N-({(1S)-5-[4-(13-{[2,4-BIS(DIHYDROXYAMINO)PHENYL]AMINO}-2,5,8,11-TETRAOXATRIDEC-1-YL)-1H-1,2,3-TRIAZOL-1-YL]-1-CARBOXYPENTYL}CARBAMOYL)-L-GLUTAMIC 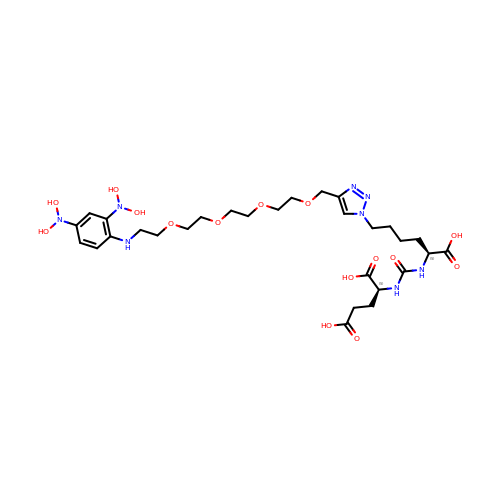ACID | C29 H46 N8 O15 | OGVHLQGCHPCUQO-ZEQRLZLVSA-N>[3x]RVVQPVIVEPIASGQGRAIKAWTGYSVSKWTASCAAAEAKVTSAITISLPNELSSERNKQLK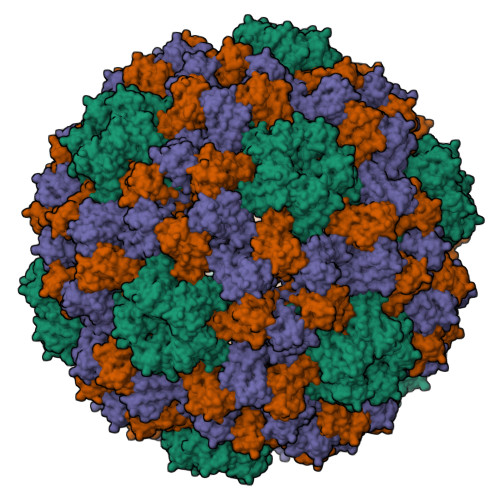VGRVLLWLGLLPSVSGTVKSCVTETQTTAAASFQVALAVADNSKDVVAAMYPEAFKGITLEQLAADLTIYLYSSAALTEGDVIVHLEVEHVRPTFDDSFTPVY The functionally conserved MON1−CCZ1 (MC1) complex serves as a guanine nucleotide exchange factor (GEF) for the RAB GTPase RAB7A and is indispensable for directing RAB7A recruitment to autophagosome or lysosomal membranes. Among RAB family members, RAB7A serves as a master regulator of late endosomal maturation, lysosomal biogenesis, and autophagosome−lysosome fusion. The spatiotemporal activation of RAB GTPases is precisely controlled by guanine nucleotide exchange factors (GEFs) that catalyze GDP−GTP exchange, and GTPase-activating proteins (GAPs) that accelerate GTP hydrolysis. In metazoans, the MON1−CCZ1 (MC1) complexes have evolved through the incorporation of an additional non-tri-longin domain (non-TLD) subunit, RMC1 (Regulator of MON1−CCZ1) in humans and Bulli in Drosophila, suggesting functional specialization in higher eukaryotes.

To address these knowledge gaps, we present the high-resolution cryo-EM structure of the human MON1A−CCZ1−RAB7AN125I (HsMCR7N125I) complex at 2.85 Å resolution, capturing RAB7A in a nucleotide-free state stabilized through unprecedented interactions with CCZ1. Due to the RAB7AN125I (the nucleotide-free mutant) exhibiting poor solubility when expressed alone, we co-expressed HsRAB7AN125I with HsMC1 in Sf9 insect cells via dual baculovirus infection, enabling efficient complex assembly. The final structure demonstrated that HsMC1 adopts a heterodimeric architecture, with MON1A and CCZ1 each comprising three tandem LDs (LD1−LD3). Inter-subunit interactions within HsMC1 are mediated by β-sheet fusion between LD1 and LD3 domains of MON1A and CCZ1, forming two continuous β-sheets that stabilize the heterodimer. Consistent with evolutionary conservation of GEF−RAB interfaces, the primary RAB7A binding sites are located within the LD1 domain of HsMC1, with MON1A contributing predominantly and CCZ1 playing a minor role. High-resolution density maps resolved key residues at the HsMC1−RAB7A interfaces (Supplementary Fig. S4a−c), involving RAB7A’s nucleotide-sensitive regions: the Switch I (N30−D44), Switch II (A65−G80), and the P-loop (G15−T22). MON1A engages RAB7A through polar contacts between its E260/E290 side chains and RAB7A R79, as well as K263 and RAB7A D82. CCZ1 contributes complementary interactions via hydrogen bonds between E41/R60 and RAB7A R69, Q70 and RAB7A Q36, and E38 and RAB7A Q67/S17. Comparative analysis of GTP-bound and HsMC1-bound RAB7A revealed large-scale rearrangements in nucleotide-sensitive regions: Switch I (19.7 Å), Switch II (6.3 Å), and P-loop (10.7 Å). Our data support a two-step nucleotide displacement model: MON1A-mediated Switch I restructure weakens GDP binding, while CCZ1-driven P-loop rearrangement disrupts Mg2+ coordination, enabling passive nucleotide exchange.

> MAAAAAGAGSGPWAAQEKQFPPALLSFFIYNPRFGPREGQEENKILFYHPNEVEKNEKIRNVGLCEAIVQFTRTFSPSKPAKSLHTQKNRQFFNEPEENFWMVMVVRNPIIEKQSKDGKPVIEYQEEELLDKVYSSVLRQCYSMYKLFNGTFLKAMEDGGVKLLKERLEKFFHRYLQTLHLQSCDLLDIFGGISFFPLDKMTYLKIQSFINRMEESLNIVKYTAFLYNDQLIWSGLEQDDMRILYKYLTTSLFPRHIEPELAGRDSPIRAEMPGNLQHYGRFLTGPLNLNDPDAKCRFPKIFVNTDDTYEELHLIVYKAMSAAVCFMIDASVHPTLDFCRRLDSIVGPQLTVLASDICEQFNINKRMSGSEKEPQFKFIYFNHMNLAEKSTVHMRKTPSVSLTSVHPDLMKILGDINSDFTRVDEDEEIIVKAMSDYWVVGKKSDRRELYVILNQKNANLIEVNEEVKKLCATQFNNIFFLD;> MATDMQRKRSSECLDGTLTPSDGQSMERAESPTPGMAQGMEPGAGQEGAMFVHARSYEDLTESEDGAASGDSHKEGTRGPPPLPTDMRQISQDFSELSTQLTGVARDLQEEMLPGSSEDWLEPPGAVGRPATEPPREGTTEGDEEDATEAWRLHQKHVFVLSEAGKPVYSRYGSEEALSSTMGVMVALVSFLEADKNAIRSIHADGYKVVFVRRSPLVLVAVARTRQSAQELAQELLYIYYQILSLLTGAQLSHIFQQKQNYDLRRLLSGSERITDNLLQLMARDPSFLMGAARCLPLAAAVRDTVSASLQQARARSLVFSILLARNQLVALVRRKDQFLHPIDLHLLFNLISSSSSFREGEAWTPVCLPKFNAAGFFHAHISYLEPDTDLCLLLVSTDREDFFAVSDCRRRFQERLRKRGAHLALREALRTPYYSVAQVGIPDLRHFLYKSKSSGLFTSPEIEAPYTSEEEQERLLGLYQYLHSRAHNASRPLKTIYYTGPNENLLAWVTGAFELYMCYSPLGTKASAVSAIHKLMRWIRKEEDRLFILTPLTY;> MTSRKKVLLKVIILGDSGVGKTSLMNQYVNKKFSNQYKATIGADFLTKEVMVDDRLVTMQIWDTAGQERFQSLGVAFYRGADCCVLVFDVTAPNTFKTLDSWRDEFLIQASPRDPENFPFVVLGIKIDLENRQVATKRAQAWCYSKNNIPYFETSAKEAINVEQAFQTIARNALKQETEVELYNEFPEPIKLDKNDRAKASAESCSC pmcThe human macrophage migration inhibitory factor (MIF) superfamily, comprised of MIF and D-dopachrome tautomerase (DDT, also called MIF-2), is broadly and constitutively expressed with involvement in proinflammatory and host antimicrobial responses. MIF and MIF-2 are highly similar in structure, with monomeric units of 114 and 117 amino acids, respectively, that form homotrimers. An evolutionarily conserved proline at the N terminus acts as the catalytic base for a tautomerization reaction of unknown biological significance in both proteins. The same site in MIF-2 is Phe100 and is also evolutionarily conserved among all MIF-2 proteins, suggesting this site plays an important role in both proteins.

The MIF-2 S62A variant was made to test this serine as a transmission conduit between Phe100 and Pro1 in MIF-2, equivalent to His62 bridging Tyr99 and Pro1 in MIF. The loss in enzymatic activity of MIF-2 S62A (13%) is qualitatively similar to that of MIF H62A (25%), relative to the activities of their respective wt proteins. Ser62 and His62 are not part of the active sites, with side chains that point into the solvent cavity or channel, respectively, and are not expected to cause any enzymatic activity loss unless each residue is involved in the transmission pathway between the allosteric and active sites. It must be noted that Ser62 interacts with Phe2, adjacent to Pro1, meaning the impact of the S62A mutation on catalysis could in part be due to loss of communication between Ser62 and Phe2 that propagates to Pro1. However, the crystal structure of S62A MIF-2 shows no evidence of alteration to the Phe2 side chain relative to that of wt-MIF-2, suggesting this factor may not have a large influence. Crystal structures of MIF variants and substrate- or inhibitor-bound complexes typically display very few differences, and consistent with this trend, the P1G and S62A variants have RMSD values of 0.30 Å and 0.32 Å with the wt-MIF-2 trimer, respectively. However, the catalytically active S62A shows a water network slightly less dense than wt-MIF-2/P1G, correlating with its modestly attenuated activity. The S62A variant displayed the weakest structural and dynamic perturbations. Consistent with its modest effect on MIF-2 chemical shifts and enzymatic activity, S62A displays R1R2 parameters that deviate least from wt-MIF-2. While the inflammatory cellular response was modestly impacted by S62A administration, it did decrease alveolar–capillary leak in the murine model, when compared with wt-MIF2.

>[3x]PFLELDTNLPANRVPAGLEKRLCAAAASILGKPADRVNVTVRPGLAMALSGSTEPCAQLSIASIGVVGTAEDNRSHSAHFFEFLTKELALGQDRILIRFFPLESWQIGKIGTVMTFL> ISLAKVGCASQIGKRKENEDRFDFAQLTDEVLYFAVYDGHGGPAAADFCHTHMEKCIMDLLPKEANLETLLTLAFLEIDKAFSSHARLSADATLLTSG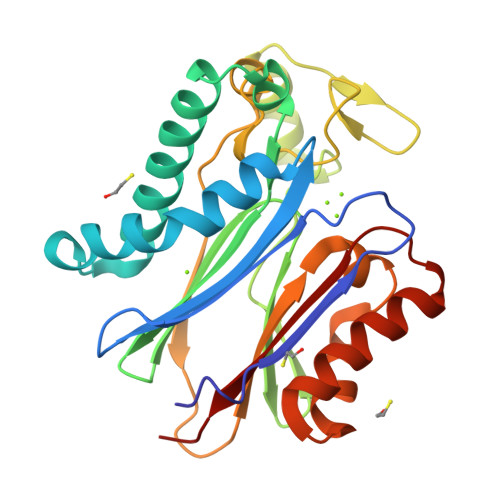TTATVALLRDGIELVVASVGDSRAILCRKGKPMKLTIDHTPERADEKERIKKCGGFVAWNQPHVNGRLAMTRSIGDLDLKTSGVIAEPETKRIKLHHADDSFLVLTTDGINFMVNSQEICDFVNQCHDPNEAAHAVTEQAIQYGTEDNSTAVVVPFGAW> GPVRLPGLAAMRQGTRLFTPEQGEDLREALRRRRGSFQTTCEVTSETTFAAARRLREKASALAALNFASAKNPGGGFLGGAQAQEEDLCRGSGLYFSLTSPQAEPYYAVNRQSHSALYTDHLIYSPQVPIFRDDAGQLLPAPVPVNIITAPAPNAGAVAQSRPEQLPQVLPTLRERARRVLGVAAWMEQTHLVLGAWGCGVFRNDPAGVARTFRELLEGEAQGAFEHVTFAVLDNHPQHPTLGAFRRELESLCLP

Despite the abundance of PARP1, most of the PAR generated by DNA damage is rapidly degraded, with a half-life of less than 1 min by poly (ADP-ribose) glycohydrolase (PARG). The radio-resistant bacterium D. radiodurans encodes a PARG homolog, DrPARG, whose expression is upregulated after radiation damage, so it might play an important role in DNA repair. Our study demonstrates that DrPARG is involved in catalyzing the breakdown of endogenous PAR and DNA repair in D. radiodurans. From observing the structural peculiarities of DrPARG, we show that although previously thought to be an obligate exo-glycohydrolase, bacterial PARG could exert both exo- and endo-glycohydrolase functions.

To determine the mechanistic basis of DrPARG-mediated ADP-ribose modification, we here solve crystal structures of DrPARG in the absence and presence of ADP-ribose. The crystal structure of DrPARG at 1.54 Å resolution reveals a typical macrodomain folding consisting of a seven-stranded β-sheet sandwiched between nine α-helices. Eleven residues (GGGFLGGAQAQ) from position 100 to 110 in the apo-form structure of DrPARG, belonging to the catalytic loop of glycohydrolase, that were not well defined in the electron density maps were omitted. The crystal structure of the space group P212121 of DrPARG contains one molecule per asymmetric unit. Upon ADP-ribose binding, as compared with the apo-form structure, that of DrPARG changes significantly. The missing 11 residues (100GGGFLGGAQAQ110) from the catalytic loop of the apo-form structure could be defined as a loop region in the ADP-ribose-bound form. As compared with the apo-form structure, the bound form structure of DrPARG showed additional secondary structures: a short β-strand (denoted β4′) following β4, extension of β5, and an α-helix (denoted α4′) preceding α4. Consistent with the thermal denaturation study, structural analysis showed that in the bound form structure, the induced α4′ helix formed more intra-molecular hydrogen bonds, especially with residues from the loop connecting β3 and α4′, whereas the equivalent region of the apo-form structure formed fewer hydrogen bonds with surrounding residues. The presence of inducible secondary structures observed from the comparison of apo- and bound-form structures confirms that conformational changes occur during ADP-ribose binding to DrPARG.>[2x]AMVFSSKSLALQAQKKILSKIASKTVANMLIDDTSSEIFDELYKVTKEHTHNKKEAHKIMKDLIKVAIKIGILYRNNQFSQEELVIVEKFRKKLNQTAMTIVS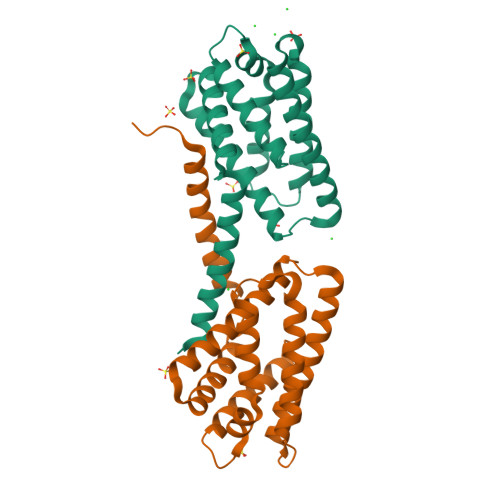FYEVEYTFDRNVLSNLLHECKDLVHELVQRHLTPRTHGRINHVFNHFADVEFLSTLYSLDGDCRPNLKRICEGINKLLDEKVL>MEIVEYPDPILRAKNKRIDIFD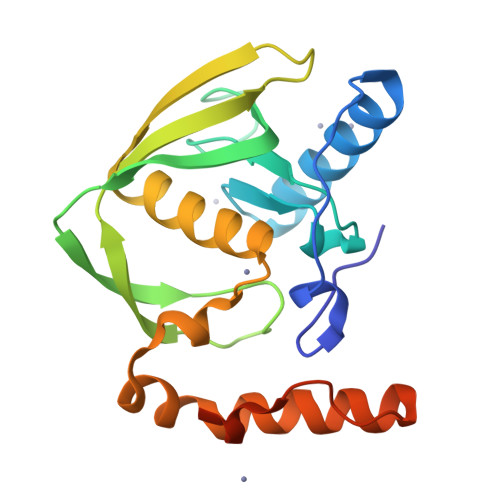ENLKNLVDAMFDVMYKTDMIGLSAPQVGLNVQLMVFNPAGEPGEGKEIVLVNPKIKKYSDKLVPFDEGCLSFPGIYAEVVRPQSVKIDARDITGERFSISLSRLPARIFQHEYDHLEGVLFFDRMTDQVLDSIREELEALEKKYEEKTGLPSPERVEARQKRKAGVGFGKR[2x]>LKCYQHGKVVTCHRDMKFCYHNAGMPFRNLKLILQGCS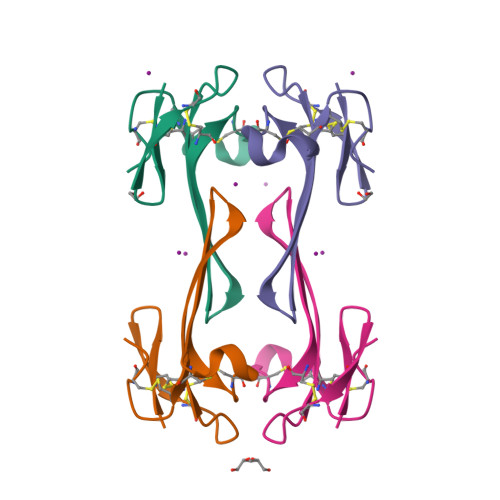SSCSETENNKCCSTDRCNK[2x]> PSKAFETLPNIYLVGPMGAGKTTVGRHLAELLGREFLDSDHEIER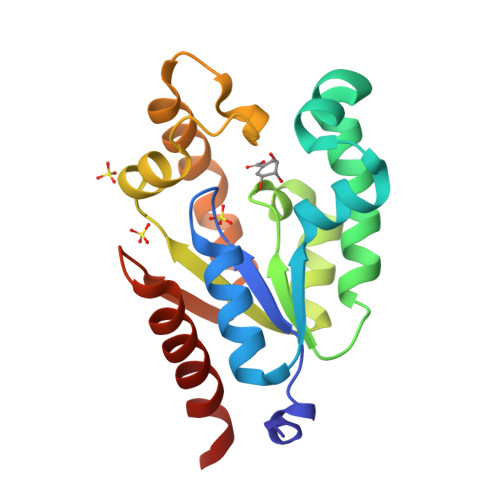KTGATIPWIFEKEGEVGFRTRETVVLNELTSRKALVLATGGGAITQAPNREFLKQRGIVVYLYTPVELQLQRTYRDKNRPLLQVENPEQKLRDLLKIRDPLYREVAHYTIETNQGAARDLAQKILQLILSNKLK> MNLIENITSEYIQTHALEFSRGFAVLTLIYEQAVQMWKMNVVYTRAGDEEPQPPIYGVKLALSTTHIKHRNWPFDFTVIDTTNNGMDPYRAD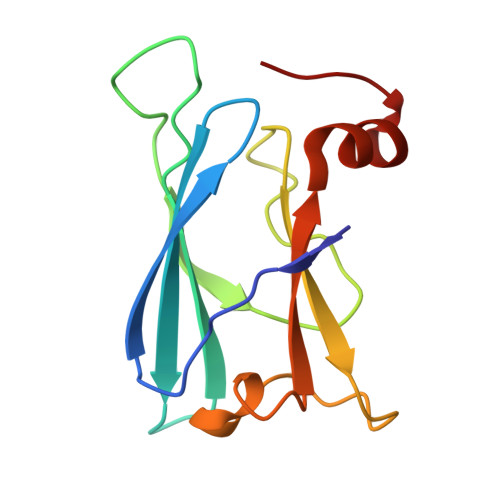DFETGRCQLYFITPEEMIQVRGVDVQ> ASYRRPSRASPTGQARKPHVGVRRLAAEYVWPGVVLVKQRKVIAFNVETKRRNRHFKLYPGENVKVSKVTNLVALCHGRVKFTHDVSR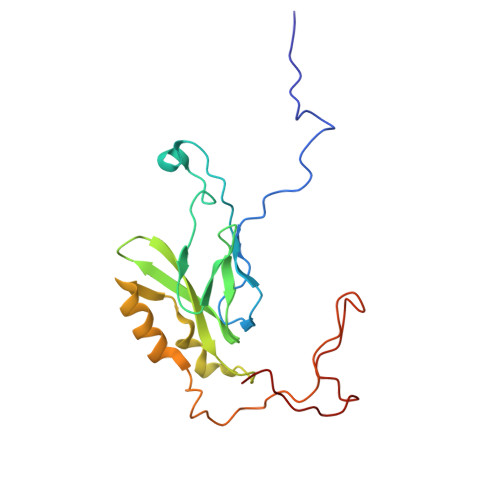DVLVVNVLPERREELLREDLWRYRTEHVRSMEENRHICFLRRKAVRMFGKELVNPPTKPPLRPFYFTKYDSWENPALPDVPQLDDD FORMAMIDE | C H3 N O | 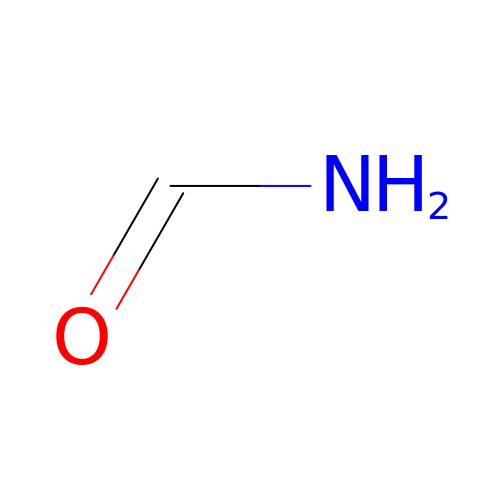ZHNUHDYFZUAESO-UHFFFAOYSA-N> MKDLVDTTEMYLRTIYELEEEGVTPLRARIAERLEQSGPTVSQTVARMERDGLVVVASDRSLQMTPTGRTLATAVMRKHRLAERLLTDIIGLDINKVHDEACRWEHVMSDEVERRLVKVLKDVSRSPFGNPIPGLDELG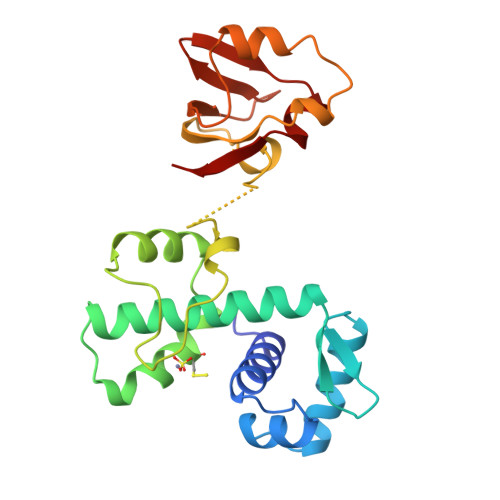VGNSDAAAPGTRVIDAATSMPRKVRIVQINEIFQVETDQFTQLLDADIRVGSEVEIVDRDGHITLSHNGKDVELLDDLAHTIRIEEL>[5x]MAHHHHHHSSGLEVLFQGPMNESVKEIPDVLKSQCGFNCLTDISHSSFNEFRQQVSEHLSWSETHDLYHDAQQAQKDNRLYEARILKRANPQLQNAVHLAILAPNAELIGYNNQFSGRASQYVAPGTVSSMFSPAAYLTELYREARNLHASDSVYYLDTRRPDLKSMALSQQNMDIELSTLSLSNELLLESIKTESKLENYTKVMEMLSTFRPSGATPYHDAYENVREVIQLQDPGLEQLNASPAIAGLMHQASLLGINASISPELFNILTEEITEGNAEELYKKNFGNIEPASLAMPEYLKRYYNLSDEELSQFIGKASNFGQQEYSNNQLITPVVNSSDGTVKVYRITREYTTNAYQMDVELFPFGGENYRLDYKFKNFYNASYLSIKLNDKRELVRTEGAPQVNIEYSANITLNTADISQPFEIGLTRVLPSGSWAYAAAKFTVEEYNQYSFLLKLNKAIRLSRATELSPTILEGIVRSVNLQLDINTDVLGKVFLTKYYMQRYAIHAETALILCNAPISQRSYDNQPSQFDRLFNTPLLNGQYFSTGDEEIDLNSGSTGDWRKTILKRAFNIDDVSLFRLLWITDHDNKDGKIKNNL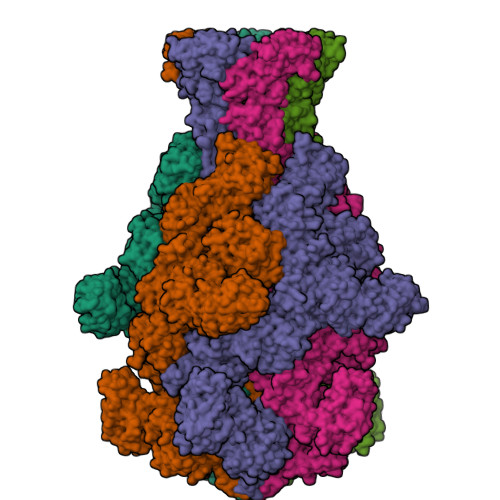KNLSNLYIGKLLADIHQLTIDELDLLLIAVGEGKTNLSAISDKQLATLIRKLNTITSWLHTQKWSVFQLFIMTSTSYNKTLTPEIKNLLDTVYHGLQGFDKDKADLLHVMAPYIAATLQLSSENVAHSVLLWADKLQPGDGAMTAEKFWDWLNTKYTPGSSEAVETQEHIVQYCQALAQLEMVYHSTGINENAFRLFVTKPEMFGAATGAAPAHDALSLIMLTRFADWVNALGEKASSVLAAFEANSLTAEQLADAMNLDANLLLQASIQAQNHQHLPPVTPENAFSCWTSINTILQWVNVAQQLNVAPQGVSALVGLDYIQSMKETPTYAQWENAAGVLTAGLNSQQANTLHAFLDESRSAALSTYYIRQVAKAAAAIKSRDDLYQYLLIDNQVSAAIKTTRIAEAIASIQLYVNRALENVEENANSGVISRQFFIDWDKYNKRYSTWAGVSQLVYYPENYIDPTMRIGQTKMMDALLQSVSQSQLNADTVEDAFMSYLTSFEQVANLKVISAYHDNINNDQGLTYFIGLSETDAGEYYWRSVDHSKFNDGKFAANAWSEWHKIDCPINPYKSTIRPVIYKSRLYLLWLEQKEITKQTGNSKDGYQTETDYRYELKLAHIRYDGTWNTPITFDVNKKISELKLEKNRAPGLYCAGYQGEDTLLVMFYNQQDTLDSYKNASMQGLYIFADMASKDMTPEQSNVYRDNSYQQFDTNNVRRVNNRYAEDYEIPSSVSSRKDYGWGDYYLSMVYNGDIPTINYKAASSDLKIYISPKLRIIHNGYEGQKRNQCNLMNKYGKLGDKFIVYTSLGVNPNNSSNKLMFYPVYQYSGNTSGLNQGRLLFHRDTTYPSKVEAWIPGAKRSLTNQNAAIGDDYATDSLNKPDDLKQYIFMTDSKGTATDVSGPVEINTAISPAKVQIIVKAGGKEQTFTADKDVSIQPSPSFDEMNYQFNALEIDGSGLNFINNSASIDVTFTAFAEDGRKLGYESFSIPVTLKVSTDNALTLHHNENGAQYMQWQSYRTRLNTLFARQLVARATTGIDTILSMETQNIQEPQLGKGFYATFVIPPYNLSTHGDERWFKLYIKHVVDNNSHIIYSGQLTDTNINITLFIPLDDVPLNQDYHAKVYMTFKKSPSDGTWWGPHFVRDDKGIVTINPKSILTHFESVNVLNNISSEPMDFSGANSLYFWELFYYTPMLVAQRLLHEQNFDEANRWLKYVWSPSGYIVHGQIQNYQWNVRPLLEDTSWNSDPLDSVDPDAVAQHDPMHYKVSTFMRTLDLLIARGDHAYRQLERDTLNEAKMWYMQALHLLGDKPYLPLSTTWSDPRLDRAADITTQNAHDSAIVALRQNIPTPAPLSLRSANTLTDLFLPQINEVMMNYWQTLAQRVYNLRHNLSIDGQPLYLPIYATPADPKALLSAAVATSQGGGWLPESFMSLWRFPHMLENARGMVSQLTQFGSTLQNIIERQDAEALNALLQNQAAELILTNLSIQDKTIEELDAEKTVLEKSKAGAQSRFDSYGKLYDENINAGENQAMTLRASAAGLTTAVQASRLAGAAADLVPNIFGFAGGGSRWGAIAEATGYVMEFSANVMNTEADKISQSETYRRRRQEWEIQRNNAEAELKQIDAQLKSLAVRREAAVLQKTSLKTQQEQTQSQLAFLQRKFSNQALYNWLRGRLAAIYFQFYDLAVARCLMAEQAYRWELNDDSARFIKPGAWQGTYAGLLAGETLMLSLAQMEDAHLKRDKRALEVERTVSLAEVYAGLPKDNGPFSLAQEIDKLVSQGSGSAGSGNNNLAFGAGTDTKTSLQASVSFADLKIREDYPASLGKIRRIKQISVTLPALLGPYQDVQAILSYGDKAGLANGCEALAVSHGMNDSGQFQLDFNDGKFLPFEGIAIDQGTLTLSFPNASMPEKGKQATMLKTLNDIILHIRYTIK> MIVKRGDVYFADLSPVVGSEQGGVRPVLVIQNDIGNRFSPTAIVAAITAQIQKAKLPTHVEIDAKRYGFERDSVILLEQIRTIDKQRLTDKITH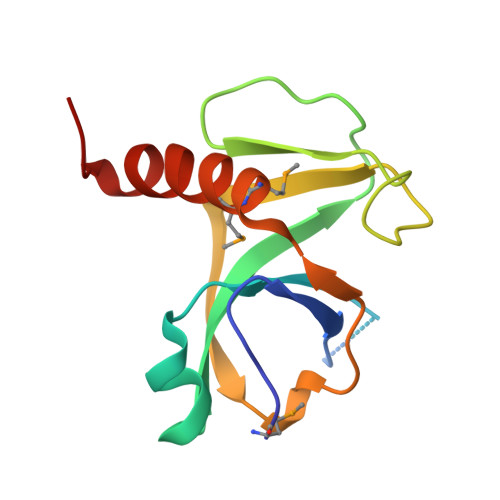LDDEMMDKVDEALQISLALIDF{6-(3,5-diaminophenyl)-1-[4-(propan-2-yl)benzyl]-1H-indol-3-yl}acetic 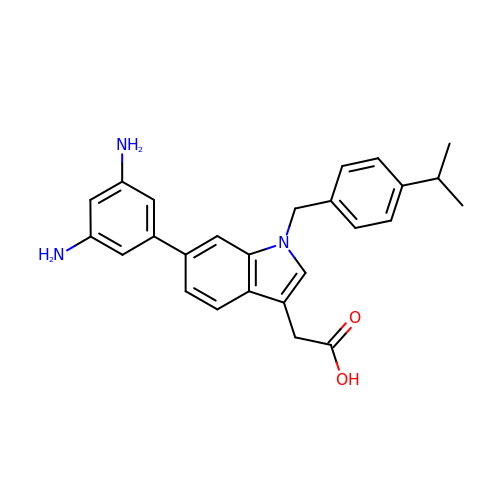acid | C26 H27 N3 O2 | VQXYFFBYBKESTK-UHFFFAOYSA-N>AGPSFWLGNETLKVPLALFALNRQRLCERLRKNPAVQAGSIVVLQGGEETQRYCTDTGVLFRQESFFHWAFGVTEPGCYGVIDVDTGKSTLFVPRLPASHATWMGKIHSKEHFKEKYAVDDVQYVDEIASVLTSQKPSVLLTLRGVNTDSGSVCREASFDGISKFEVNNTILHPEIVECRVFKTDMELEVLRYTNKISSEAHREVMKAVKVGMKEYELESLFEHYCYSRGGMRHSSYTCICGSGENSAVLHYGHAGAPNDRTIQNGDMCLFDMDGEYYCFASDITCSFPANGKFTADQKAVYEAVLRSSRAVMGAMKPGVWWPDMHRLADRIHLEELAHMGILSGSVDAMVQAHLGAVFMPHGLGHFLGIDVHDVGGYPEGVERIDEPGLRSLRTARH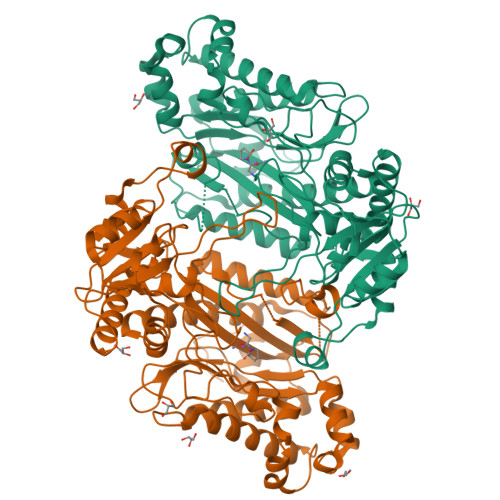LQPGMVLTVEPGIYFIDHLLDEALADPARASFLNREVLQRFRGFGGVRIEEDVVVTDSGIELLTCVPRTVEEIEACMAGCDKAFTP[2x]> DFRCPTTWSASKLYCYKPFKEKKTWIEAERFCAKQAENGHLVSIGSAAEADFLDLVIVVNFDKQRYRAWTGLTERNLKWTNGASVSYENLYEPYIRKCF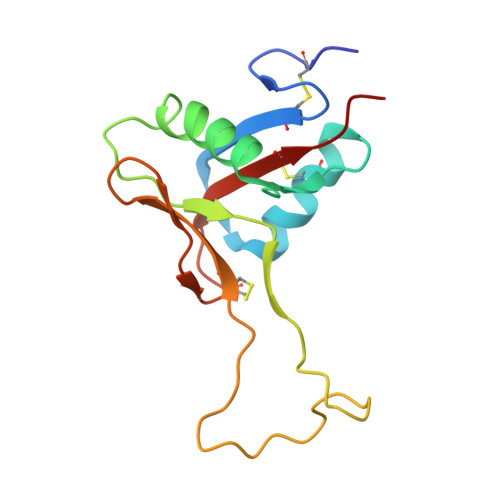VVQPWEGKSKWYKADCEEKNAFLCKFPKPH1-[(3S)-5-PHENYL-3-THIOPHEN-2-YL-3H-1,4-BENZODIAZEPIN-2-YL]AZETIDIN-3-OL 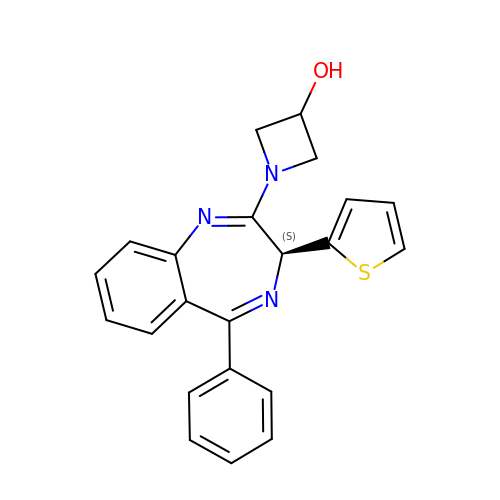| C22 H19 N3 O S | BKSGACYTXOQQNI-OAQYLSRUSA-N> SRANDAPIVLLHGFTGWGREEMFGFKYWGGVRGDIEQWLNDNGYRTYTLAVGPL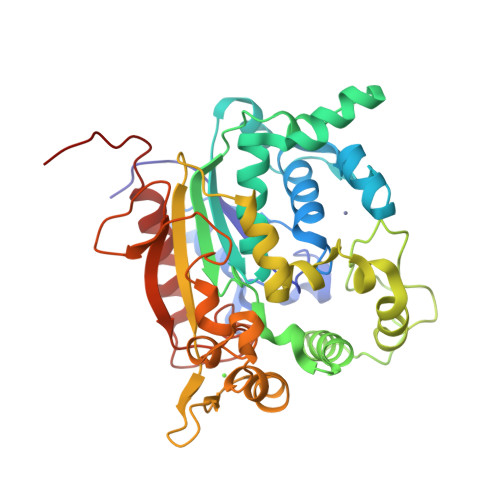SSNWDRACEAYAQLVGGTVDYGAAHAAKHGHARFGRTYPGLLPELKRGGRIHIIAHSQGGQTARMLVSLLENGSQEEREYAKAHNVSLSPLFEGGHHFVLSVTTIATPHDGTTLVNMVDFTDRFFDFQKFVLKAAAVASNVPYTSQVYDFKLDQWGLRRQPGESFDQYFERLKRSPVWTSTDTARYDLSVPGAEKLNQWVKASPNTYYLSFATERTYRGALTGNYYPELGMNAFSAVVCAPFLGSYRNATLGIDDRWLENDGIVNAFSMNGPKRGSTDRIVPYDGTIKKGVWNDMGTYNVDHLEVIGVDPNPLFDIRAFYLRLAEQLASLQPHHHHHH> MPKPINVRVTTM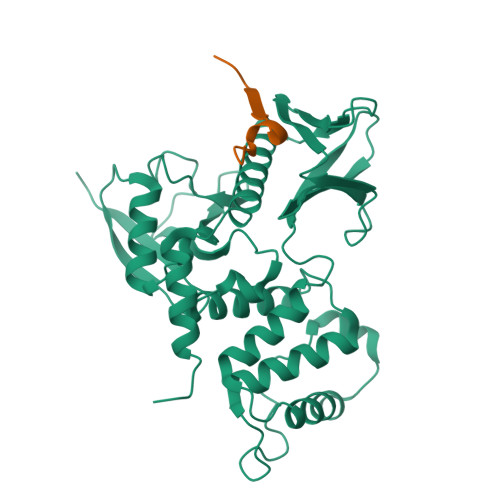DAELEFAIQPNTTGKQLFDQVVKTVGLREVWFFGLQYVDSKGYSTWLKLNKKVTQQDVKKENPLQFKFRAKFFPEDVSEELIQEITQRLFFLQVKEAILNDEIYCPPETAVLLASYAVQAKYGDYNKEIHKPGYLANDRLLPQRVLEQHKLTKEQWEERIQNWHEEHRGMLREDSMMEYLKIAQDLEMYGVNYFEIKNKKGTELWLGVDALGLNIYEHDDKLTPKIGFPWSEIRNISFNDKKFVIKPIDKKAPDFVFYAPRLRINKRILALCMGNHELYMRRRKPDTIEVQQMKAQARVDSSGAA;> RRRTGTYGVLAAWRRL OLEIC ACID | C18 H34 O2 | 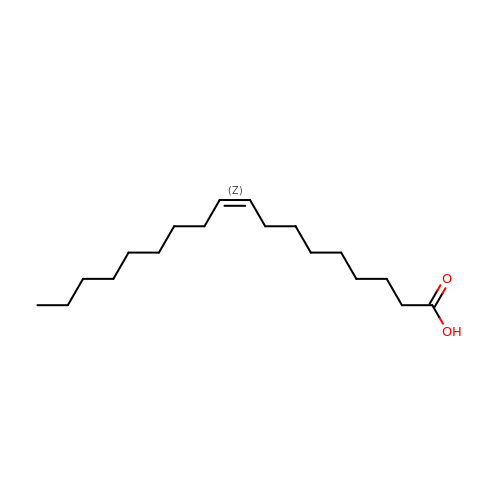ZQPPMHVWECSIRJ-KTKRTIGZSA-N> DKAEAFLEAARSNDTEEIRRLLSEGLDPNTRHRLGWTALMVAAMNTQHNVVKLLLDAGADPNLGDGFSSVYDTAREKSLHSLEVLVSREDEFSSRLSSRASFRGCSALHYAALADDLQTVRLLLDAGADPSLKNDLGHTPLSYARDGELSAVLRDAQDTFAEAQRKREAEERRKFPLERRLKEHIIGQEGAINTVASAIRRKENGWYDEEHPLVFLFLGSSGIGKTELAKQVARYMHKDIKKGFIRMDMSEFQEKHEVAKFIGSPPGYVGHDEG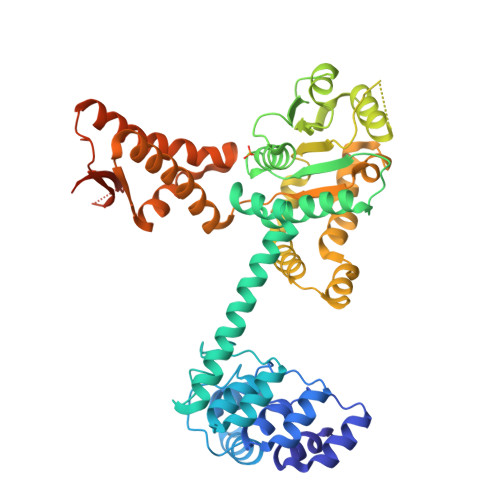GQLTKQLKQSPSAVVLFDEVEKAHPDVLTVMLQLFDEGRLTDGKGKTIECKDAIFIMTSNAASDEIAQHALQLRQEAQEQSRRRLAENLDDVQKSENITISNTFKEQVIRPILKAHFRRDEFLGRINEIVYFLPFCHSELLQLVSRELHYWAKKAKQRHNITLLWERPVLELLVKGYNLHYGARSIKHEVERRVVNQLAAAFEQELLPKGCTLRLTVDRDSQHTDGAPVLRLELLQEDKTSRKLEIQPPLNPQDTAHTPRKH[(2~{R},3~{S},4~{S},5~{R})-3,4-bis(oxidanyl)-5-[3-[4-(2-phenylethyl)-1,2,3-triazol-1-yl]propyl]oxan-2-yl]methyl ~{N}-[(2~{S})-2-azanyl-4-methyl-pentanoyl]sulfamate | C25 H39 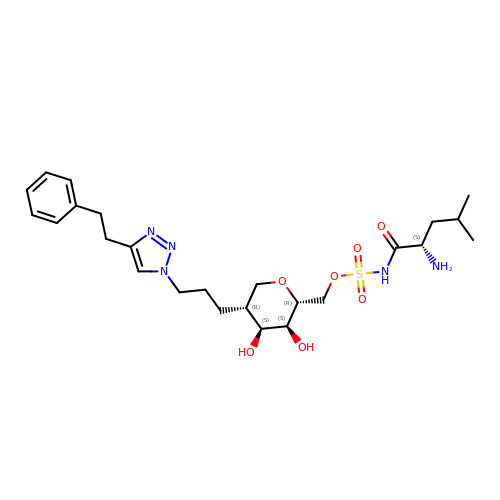N5 O7 S | OGPNUIVQHZNEJO-MENZVKOBSA-N>MCEKYDVAIIGGGVIGSSVAHFLAERGHKVAIVEKQSIASEASKAAAGLLGVQAEWDAYNPLFELARESRAIFPQLAAVLREKTGVDIGYEEKGIYRIAQNEDEKERILHIMDWQQKTGEDSYFLTGDHVREKEPYLSESIIGAVYYPKDGHVIAPELTKAFAHSAAISGADIYEQTEVFDIRIENNKVTGVITSEGIVTCEKVVIAGGSWSTKLLSYFHRDWGTYPVKGEVVAVRSRKQLLKAPIFQERFYITPKRGGRYVIGATMKPH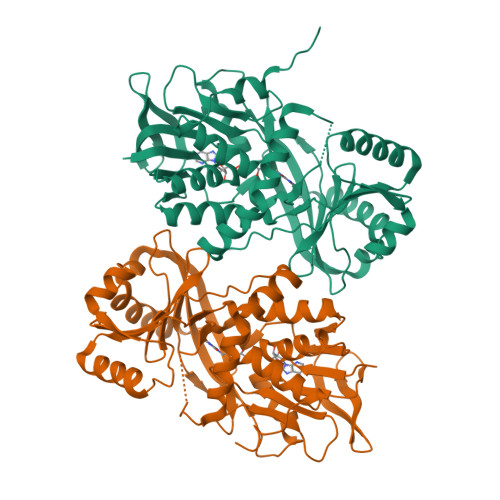TFNKTVQPESITSILERAYTILPALKEAEWESTWAGLRPQSNHEAPYMGEHEEIKGLYACTGHYRNGILLSPISGQYMADLIEGKQENHLLDSLLSRRVLEHHHHHH[2x]> MSNKEKNASETRKAYTTKMIPRSHDRMKLLGNFMDYLMDGTPIFFELWNQFGGGIDRDIISGTANKD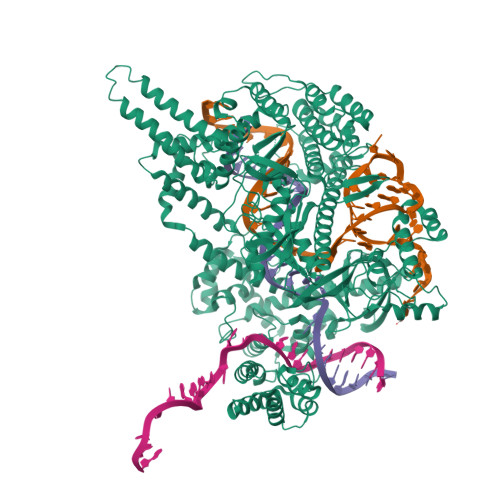KISDDLLLAVNWFKVMPINSKPQGVSPSNLANLFQQYSGSEPDIQAQEYFASNFDTEKHQWKDMRVEYERLLAELQLSRSDMHHDLKLMYKEKCIGLSLSTAHYITSVMFGTGAKNNRQTKHQFYSKVIQLLEESTQINSVEQLASIILKAGDCDSYRKLRIRCSRKGATPSILKIVQDYELGTNHDDEVNVPSLIANLKEKLGRFEYECEWKCMEKIKAFLASKVGPYYLGSYSAMLENALSPIKGMTTKNCKFVLKQIDAKNDIKYENEPFGKIVEGFFDSPYFESDTNVKWVLHPHHIGESNIKTLWEDLNAIHSKYEEDIASLSEDKKEKRIKVYQGDVCQTINTYCEEVGKEAKTPLVQLLRYLYSRKDDIAVDKIIDGITFLSKKHKVEKQKINPVIQKYPSFNFGNNSKLLGKIISPKDKLKHNLKCNRNQVDNYIWIEIKVLNTKTMRWEKHHYALSSTRFLEEVYYPATSENPPDALAARFRTKTNGYEGKPALSAEQIEQIRSAPVGLRKVKKRQMRLEAARQQNLLPRYTWGKDFNINICKRGNNFEVTLATKVKKKKEKNYKVVLGYDANIVRKNTYAAIEAHANGDGVIDYNDLPVKPIESGFVTVESQVRDKSYDQLSYNGVKLLYCKPHVESRRSFLEKYRNGTMKDNRGNNIQIDFMKDFEAIADDETSLYYFNMKYCKLLQSSIRNHSSQAKEYREEIFELLRDGKLSVLKLSSLSNLSFVMFKVAKSLIGTYFGHLLKKPKNSKSDVKAPPITDEDKQKADPEMFALRLALEEKRLNKVKSKKEVIANKIVAKALELRDKYGPVLIKGENISDTTKKGKKSSTNSFLMDWLARGVANKVKEMVMMHQGLEFVEVNPNFTSHQDPFVHKNPENTFRARYSRCTPSELTEKNRKEILSFLSDKPSKRPTNAYYNEGAMAFLATYGLKKNDVLGVSLEKFKQIMANILHQRSEDQLLFPSRGGMFYLATYKLDADATSVNWNGKQFWVCNADLVAAYNVGLVDIQKDFKKKLEHHHHHH> MELAALCRWGLLLALLPPGAASTQVCTGTDMKLRLPA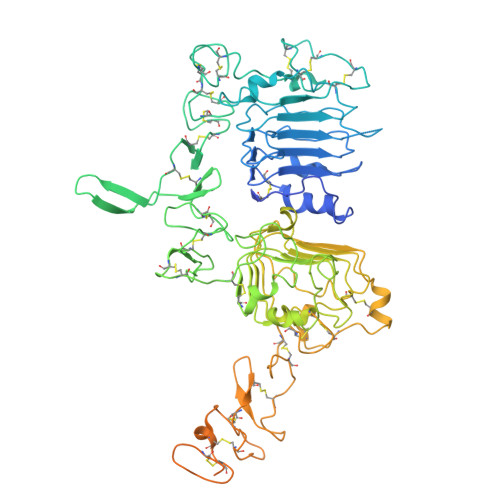SPETHLDMLRHLYQGCQVVQGNLELTYLPTNASLSFLQDIQEVQGYVLIAHNQVRQVPLQRLRIVRGTQLFEDNYALAVLDNGDPLNNTTPVTGASPGGLRELQLRSLTEILKGGVLIQRNPQLCYQDTILWKDIFHKNNQLALTLIDTNRSRACHPCSPMCKGSRCWGESSEDCQSLTRTVCAGGCARCKGPLPTDCCHEQCAAGCTGPKHSDCLACLHFNHSGICELHCPALVTYNTDTFESMPNPEGRYTFGASCVTACPYNYLSTDVGSCTLVCPLHNQEVTAEDGTQRCEKCSKPCARVCYGLGMEHLREVRAVTSANIQEFAGCKKIFGSLAFLPESFDGDPASNTAPLQPEQLQVFETLEEITGYLYISAWPDSLPDLSVFQNLQVIRGRILHNGAYSLTLQGLGISWLGLRSLRELGSGLALIHHNTHLCFVHTVPWDQLFRNPHQALLHTANRPEDECVGEGLACHQLCARGHCWGPGPTQCVNCSQFLRGQECVEECRVLQGLPREYVNARHCLPCHPECQPQNGSVTCFGPEADQCVACAHYKDPPFCVARCPSGVKPDLSYMPIWKFPDEEGACQPCPINCTHSCVDLDDKGCPAEQRASPLTSIISAVVGILLVVVLGVVFGILIKRRQQKIRKYTMRRLLQEGGSENLYFQGGGSAQLEKELQALEKENAQLEWELQALEKELAQSNSLEVLFQ>[2x]MEEPEEPADSGQSLVPVYIYSPEYVSMCDSLAKIPKRASMVHSLIEAYALHKQMRIVKPKVASMEEMATFHTDAYLQ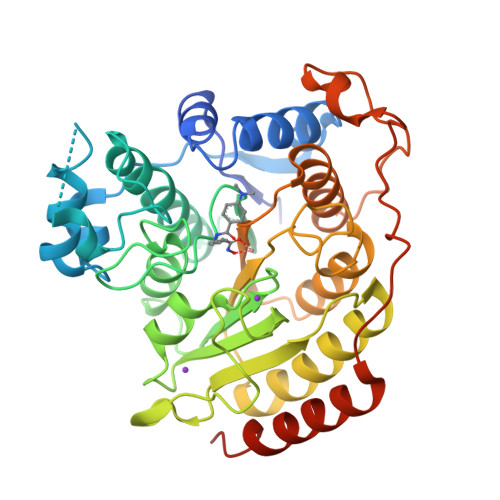HLQKVSQEGDDDHPDSIEYGLGYDCPATEGIFDYAAAIGGATITAAQCLIDGMCKVAINWSGGWHHAKKDEASGFCYLNDAVLGILRLRRKFERILYVDLDLHHGDGVEDAFSFTSKVMTVSLHKFSPGFFPGTGDVSDVGLGKGRYYSVNVPIQDGIQDEKYYQICESVLKEVYQAFNPKAVVLQLGADTIAGDPMCSFNMTPVGIGKCLKYILQWQLATLILGGGGYNLANTARCWTYLTGVILGKTLSSEIPDHEFFTAYGPDYVLEITPSCRPDRNEPHRIQQILNYIKGNLKHVVIEGRGSHHHHHH> MGEPRSQPPVE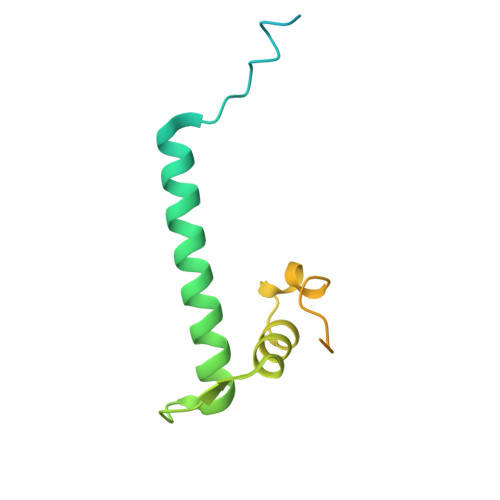RPPTAETFLPLSRVRTIMKSSMDTGLITNEVLFLMTKCTELFVRHLAGAAYTEEFGQRPGEALKYEHLSQVVNKNKNLEFLLQIVPQKIRVHQFQEMLRLNRSAGSDDDDDDDDDDDEEESESESESDE>GLFDIVKKIAGHIVSSI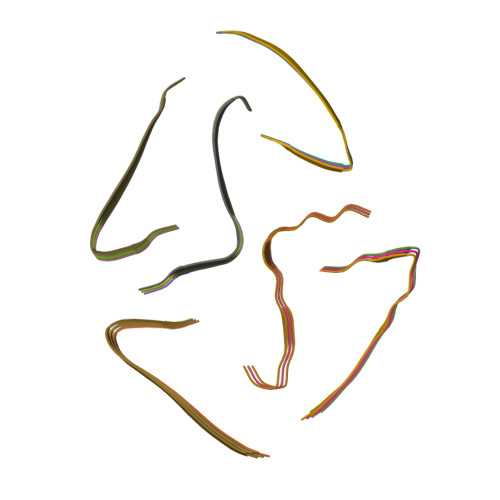[18x]> MVPPDKRSFREEHRIRGYEVSPDQRATIVTVANLLQEVAGNHAVGMWGRTDEGFASLPSMKDLLFVMTRLQVRMYEYPKWGDVVAVETYFTEEGRLAFRREWKLMDVATGKLLGAGTSTWVTINTATRRLSKLPEDVRKRFLRFAPPSSVHILPPEETKKKLQDMELPGQVQSAQQVARRADMDMNGHINNVTYLAWTLESLPERVMSGGYKMQEIELDFKAECTAGNAIEAHCNPLDDHSASFVGPAPANGNGNGHAAEPAADSAPLYFLSMLQKCDENGCTELVRARTTWSRTLEGAKPAPPPLSELSAAQGTGENLYFQGSGGGGSDYKDDDDKGTGRSRLEH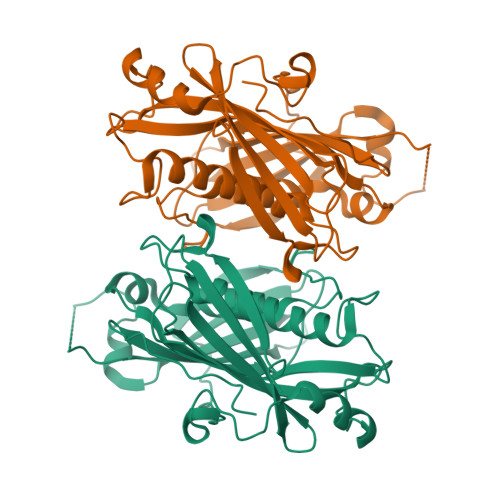HHHHH>MEESRESPAEHGYYMPAEWDSHAQTWIGWPERQDNWRHNALPAQRVFAGVAKAISKFEPVTVCASPAQWENARKQLPEDIRVVEMSMNDSWFRDSGPTFIVRKRPVKLSSLNRNIAGIDWNFNAWGGANDGCYNDWSHDLLVSRKILALERIPRFQHSMILEGGSIHVDGEGTCLVTEECLLNKNRNPHMSKEQIEEELKKYLGVQSFIWLPRGLYGDEDTNGHIDNMCCFARPGVVLLSWTDDETDPQYERSVEALSVLSNSIDA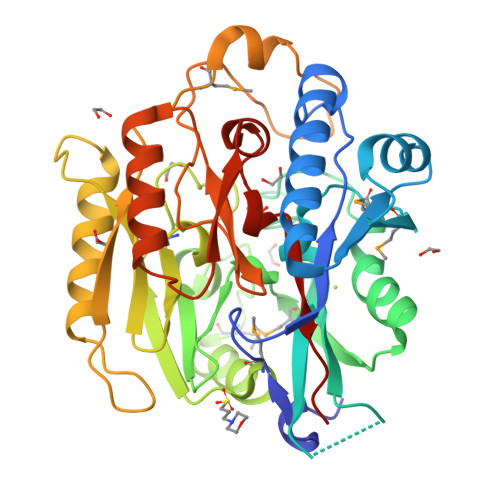RGRKIQVIKLYIPEPLYMTEEESSGITQDGEAIPRLAGTRLAASYVNFYIANGGIIAPQFGDPIRDKEAIRVLSDTFPHHSVVGIENAREIVLAGGNIHCITQQQPAEPTSVAENGH[2x]pteridine-2,4(1H,3H)-dione 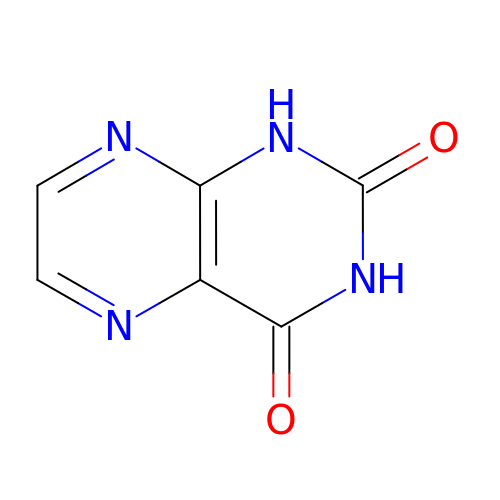| C6 H4 N4 O2 | UYEUUXMDVNYCAM-UHFFFAOYSA-N>[2x]MVPISPIETVPVKLKPGMDGPKVKQWPLTEEKIKALVEICTEMEKEGKISKIGPENPYNTPVFAIKKKDSTKWRKLVDFRELNKRTQDFWEVQLGIPHPAGLKQKKSVTVLDVSAAFYSVPLDKDFRKYTAFTIPSINNETPGIRYQYNVLPMGWKGSPALLQSSMTKILEPFRKQNPDIVIYQYMDDLYVGSDLEIGQHRTKIEELRQHLLRWGFTTPDKKHQKEPPFLWMGYELHPDKWTVQPIVLPEKDSWTVNDIQKLVGKLNWASQIYAGIKVRQLSKLLRGTKALTEVVPLTEEAELELAENREILKEPVHGVYYDPSKDLIAEIQKQGQGQWTYQIYQEPFKNLKTGKYARMKGAHTNDVKQLTEAVQKIATESIVIWGKTPKFKLPIQK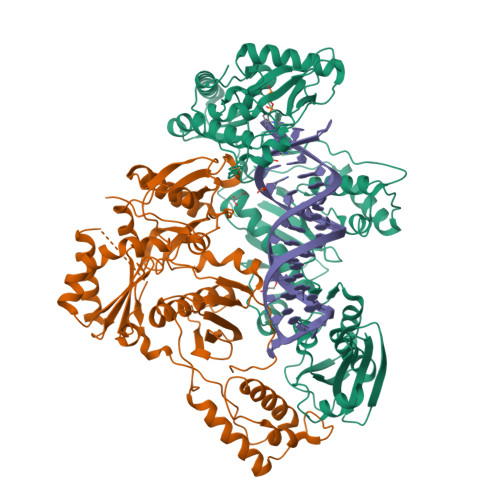ETWEAWWTEYWQATWIPEWEFVNTPPLVKLWYQLEKEPIIGAETFYVDGAANRETKLGKAGYVTDRGRQKVVPLTDTTNQKTELQAIHLALQDSGLEVNIVTDSQYALGIIQAQPDKSESELVSQIIEQLIKKEKVYLAWVPAHKGIGGNEQVDKLVSAG;>[2x]MAHHHHHHALEVLFQGPISPIETVPVKLKPGMDGPKVKQWPLTEEKIKALVEICTEMEKEGKISKIGPENPYNTPVFAIKKKDSTKWRKLVDFRELNKRTQDFWEVQLGIPHPAGLKQKKSVTVLDVGDAYFSVPLDKDFRKYTAFTIPSINNETPGIRYQYNVLPQGWKGSPAIFQSSMTKILEPFRKQNPDIVIYQYMDDLYVGSDLEIGQHRTKIEELRQHLLRWGFTTPDKKHQKEPPFLWMGYELHPDKWTVQPIVLPEKDSWTVNDIQKLVGKLNWASQIYAGIKVRQLSKLLRGTKALTEVVPLTEEAELELAENREILKEPVHGVYYDPSKDLIAEIQKQGQGQWTYQIYQEPFKNLKTGKYARMKGAHTNDVKQLTEAVQKIATESIVIWGKTPKFKLPIQKETWEAWWTEYWQATWIPEWEFVNTPPLVKLWYQ> GRCYKSI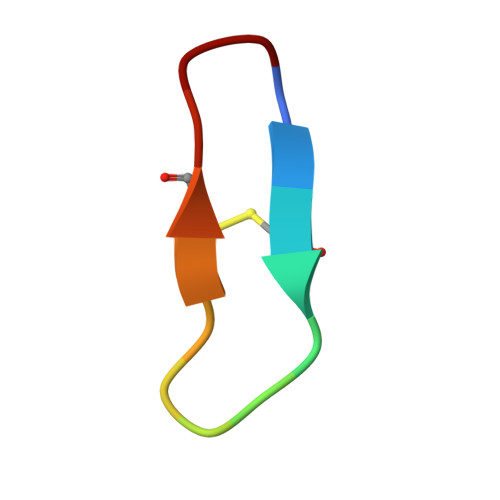PPICFPD>[3x]EKIKICLQKQVNSSFSLHNGFGGNLYATEEKRMFELVKPKAGASVLNQSTWIGFGDSRTDKSNSAFPRSADVSAKTADKFRFLSGGSLMLSMFGPPGKVDYLYQGCGKHKVFYEGVNWSPHAAINCYRKNWTDIKLNFQKNIYELASQSHCMSLVNALDKTIPLQVTAGTAGNCNNSFLKNPALYTQEVKPSENKCGKENLAFFTLPTQFGTYECKLHLVASCYFIYDSKEVYNKRGCDNYFQVIYDSFGKVVGGLDNRVSPYTGNSGDTPTMQCDMLQLKPGRYSVRSSPRFLLMPERSYCFDMKEKGPVTAVQSIWGKGRESDYAVDQACLSTPGCMLIQKQKPYIGEADDHHGDQEMRELLSGLDYEARCISQSGWVNETSPFTEKYLLPPKFGRCPLAAKEESIPKIPDGLLIPTSGTDTTVTKPKSR;>IFGI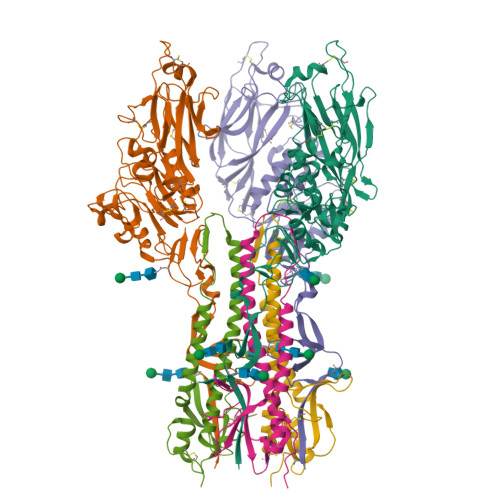DDLIIGVLFVAIVETGIGGYLLGSRKESGGGVTKESAEKGFEKIGNDIQILKSSINIAIEKLNDRISHDEQAIRDLTLEIENARSEALLGELGIIRALLVGNISIGLQESLWELASEITNRAGDLAVEVSPGCWIIDNNICDQSCQNFIFKFNETAPVPTIPPLDTKIDLQ[3x]>[4x]KPQVTILATGGTIAGSGESSVKSSYSAGAVTVDKLLAAVPAINDLAT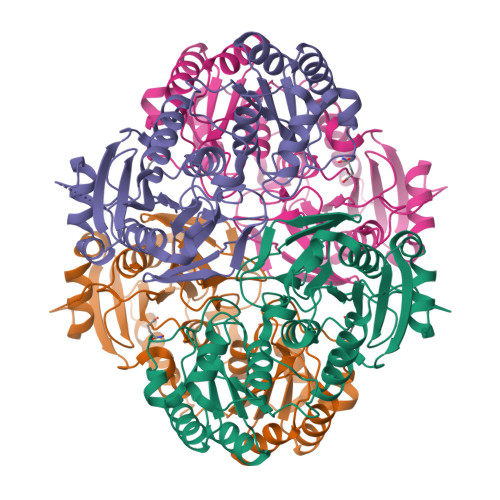IKGEQISSIGSQEMTGKVWLKLAKRVNELLAQKETEAVIITHGTDTMEETAFFLNLTVKSQKPVVLVGAMRPGSSMSADGPMNLYNAVNVAINKASTNKGVVIVMNDEIHAAREATKLNTTAVNAFASPNTGKIGTVYYGKVEYFTQSVRPHTLASEFDISKIEELPRVDILYAHPDDTDVLVNAALQAGAKGIIHAGMGNGNPFPLTQNALEKAAKSGVVVARSSRVGSGSTTQEAEVDDKKLGFVATESLNPQKARVLLMLALTKTSDREAIQKIFSTY N-[(2S)-2-(diethylamino)propyl]-2-[(2S)-2-(methylcarbamoyl)azetidin-1-yl]-6-[5-(thiophen-2-yl)pyrazolo[1,5-a]pyrimidin-3-yl]pyridine-4-carboxamide | C28 H34 N8 O2 S | 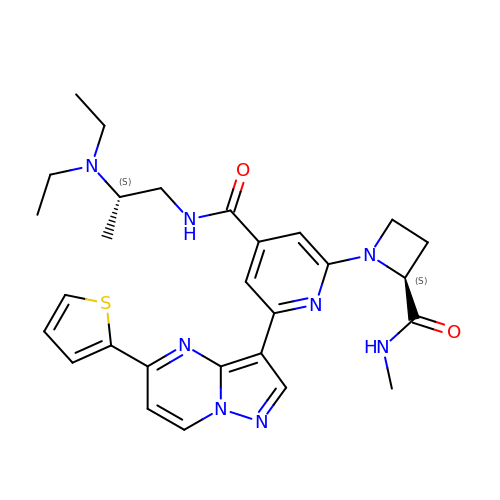BKSPZDICBZFRLV-MBSDFSHPSA-N>RADPDPMKNTCKLLVVADHRFYRYMGRGEESTTTNYLIELIDRVDDIYRNTAWDNAGFKGYGIQIEQIRILKSPQEVKPGEKHYNMAKSYPNEEKDAWDVKMLLEQFSFDIAEEASKVCLAHLFTYQDFDMGTLGLAYVGSPRANSHGGVCPKAYYSPVGKKNIYLNSGLTSTKNYGKTILTKEADLVTTHELGHNFGAEHDPDGLAECAPNEDQGGKYVMYPIAVSGDHENNKMFSQCSKQSIYKTI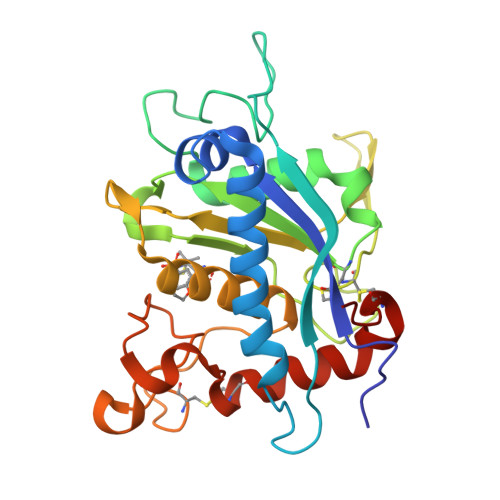ESKAQECFQERSNKV[2x]>NNNGACUUAAGUCX[2x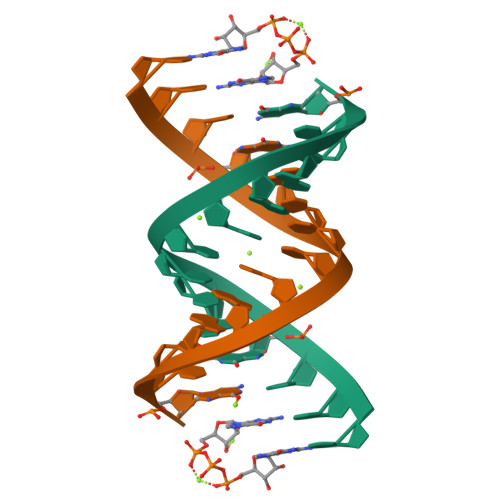]>MESLPVIAAPSMWTRPQIKDFKEKIQQDADSVITVGRGEVVTVRVPTHEEGSYLFWEFATDNYDIGFGVYFEWTDSPNTAVSVHVSESSDDDEEEEENIGCEEKAKKNANKPLLDEIVPVYRRDCHEEVYAGSHQYPGRGVYLLKFDNSYSLWRSKSVYYRVYYTR[2x];>[2x]GAMGPVYKDLEIDVCNTPPPECINDLLKS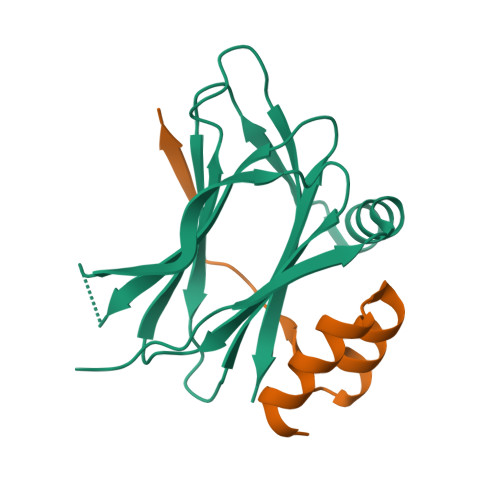VDSEEIREYCKKKKWIIPEIPTNIERAMNQ> VMVKGPG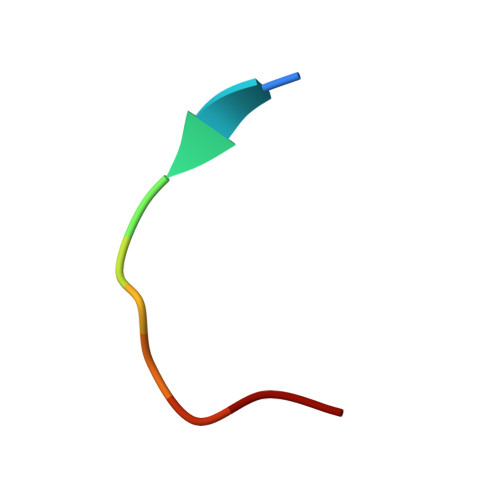PGR> MSVPADTTSPSPALDVFPSASIAPV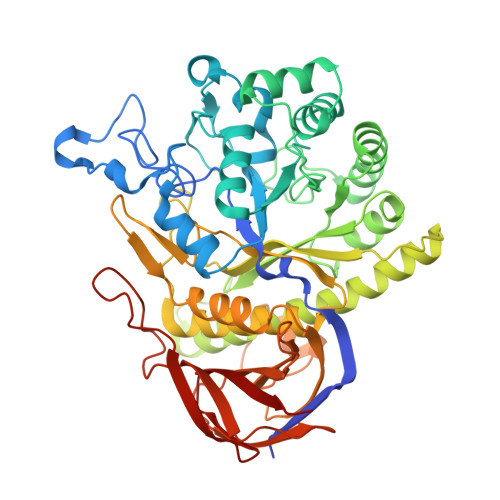SPYIFSGFLEHLGRCIYGGILPATRTTFPHTPRVPCPDAQFTETPRELLTPEGFRVDVLEVLRDELRVPLVRWPGGNYVSSYNWKDGVGPKEARKRRPELAWGGEESNVFGTDEFIAWCRVAKIEPYIVFNMGTGTLEDALHWIEYCNGTGDTYYANLRRQNTGRDEPHNVKYWALGNEVWGEWQVGQQTASAYATKARQWAHAIRLVDPSVVLVGCGETGVDHWDGVVLDELVDKVELHSIHLYTGFGPRDRSQVDKEYGRGVYGPDAAEYSIEVCKGLINKARFARNVSKPIKIAFDEYGVWDETVGTPQNGLEQFYNFADALAMASWLNVFIRQADVVDIACIAQSVNVISPLITSPTGLFRQTIYWPLYLFSRYMRDGIAVRVALESPTFAGETLPQWIASVKGRPKDLDASAVLHVDPGTSARSLRVAVVNRSEHASYEVPIRIAFERVGVQVEVHELWHQDVHARNGWGKEDEVSVKTRTERWNGRWTFREHSFTLLVLELPQ> MGSDKIHHHHHHMIRPEYLRVLRKIYDRLKNEKVNWVVTGSLSFALQGVPVEVHDIDIQTDEEGAYEIERIFSEFVSKKVRFSSTEKICSHFGELIIDGIKVEIMGDIRKRLEDGTWEDPVDLNKYKRFVETHGMK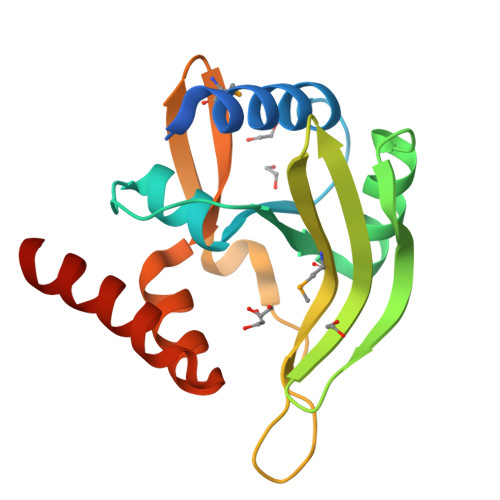IPVLSLEYEYQAYLKLGRVEKAETLRKWLNERKG Enhanced ABA levels elicited in response to drought are perceived by the PYR/PYL/RCAR family of ABA receptors and the clade A subfamily of protein phosphatases type 2C (PP2Cs), which act as necessary ABA co-receptors in ternary complexes. In the resting state, PYLR/PYL/RCAR receptors display an open ABA binding cavity flanked by two highly conserved loops, named as gate/CL2/β3-β4 loop and latch/CL3/β5-β6 loop. Specifically, both gate and latch loops define a surface that enables the receptor to dock into the PP2C active site. The formation of receptor-ABA-phosphatase complexes causes the dissociation of different PP2C-SnRK2 complexes and abolishes PP2C-mediated inhibition of the SnRK2s, triggering ABA response.

Further work was focused on N-benzyl-1,4-dimethyl-2-oxo-1,2-dihydroquinoline-6-sulfonamide because it showed in vitro activity. This compound was named as “sulfobactin” (SB) to highlight the arrangement of the sulfonamide moiety (see below). As a first step to improve binding of SB to CsPYL1, we determined and compared the crystal structure of CsPYL1-SB-HAB1 and CsPYL1-QB-HAB1 complexes. The gate and latch loops of CsPYL1 display a closed conformation that fits into the active site of the HAB1 phosphatase. Both ternary complexes yield isomorphous crystals whose molecular structure was almost identical to the previously reported CsPYL1-ABA-HAB1 complex. SB and QB display a “U”-shaped conformation into the ligand-binding pocket of the receptor. However, superimposition of the structures of the CsPYL1-SB-HAB1 and CsPYL1-QB-HAB1 ternary complexes reveals a shallower insertion of SB in the ABA binding pocket with respect to that observed for QB. This may be explained by the different orientation in SB and QB of the SO2 group, which contains one oxygen atom that shows similar position in both compounds and interacts through a water bridge with both Asn196 and the backbone carbonyl of His89, whereas the other oxygen is located in different position in SB and QB. Thus, in the QB complex, this latter oxygen forms a hydrogen bond with Arg108, whereas in the SB complex it produces steric hindrance with the Val110 side chain of CsPYL1. This difference in SO2 coordination may explain the reduced activity of SB against dimeric ABA receptors, compared to QB. Recently, opabactin has been described as a powerful ABA agonist and a key feature for its enhanced interaction with ABA receptors in the presence of a carboxylate group that interacts with a conserved Lys residue in the ABA binding pocket. Both CsPYL1-SB-HAB1 and CsPYL15m-SB-HAB1 complexes lack such interaction of the agonist with the conserved Lys88 residue of the receptor; rather, the structures show that the hydrophobic CH2 of the SB linker faces a water-filled cavity harboring the side-chain NH3+ of Lys88 (middle and right).

> MNNNKAEADTSSSMADPETRPTYTTHHLAIPSGVTQDEFDELKQSVVEFHTYQLSQNQCSSLLAQRIRAPNDVVWSIVRRFDQPQTYKHFIKSCSVSDNFTMAVGSTRDVNVISGLPAATSTERLDILDDDRQVTGFSIIGGEHRLRNYRSVTSVHGFNRDGAICTVVLESYVVDVPEGNTEEDTRLFADTVVKLNLQKLVSVAESQVI;> RSVYELDCIPLWGTVSIQGNRSEMEDAFAVSPHFLKLPIKMLMGDHEGMSPSLTHLTGHFFGVYDGHGGHKVADYCRDRLHFALAEEIERIKDELCKRNTGEGRQVQWDKVFTSCFLTVDGEIEGKIGRAVVGSSDKVLEAVASETVGSTAVVALVCSSHIVVSNCGDSRAVLFRGKEAMPLSVDHKPDREDEYARIENAGGKVIQWQGARVFGVLAMSRSIGDRYLKPYVIPEPEVTFMPRSREDECLILASDGLWDVMNNQEVCEIARRRILMWHKKNGAPPLAERGKGIDPACQAAADYLSMLALQKGSKDNISIIVIDLKAQR>MTTVMKFGGTSVGSGERIRHVAKIVTKRKKEDDDVVVVVSAMSEVTNALVEISQQALDVRDIAKVGDFIKFIREKHYKAIEEAIKSEEIKEEVKKIIDSRIEELEKVLIGVAYLGELTPKSRDYILSFGERLSSPILSGAIRDLGEKSIALEGGEAGIITDNNFGSARVKRLEVKERLLPLLKEGIIPVVTGFIGTTEEGYITTLGRGGSDYSAALIGYGLDADIIEIWTDVSGVYTTDPRLVPTARRIPKLSYIEAMELAYFGAK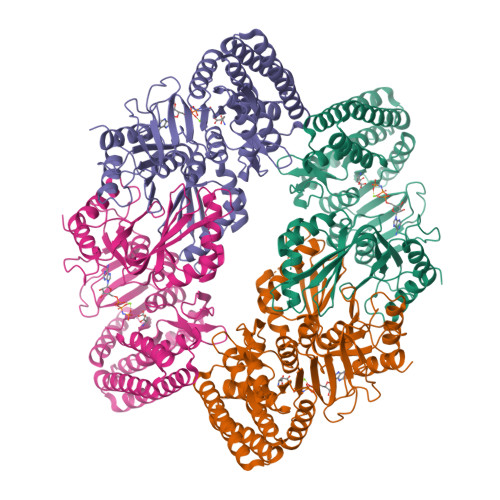VLHPRTIEPAMEKGIPILVKNTFEPESEGTLITNDMEMSDSIVKAISTIKNVALINIFGAGMVGVSGTAARIFKALGEEEVNVILISQGSSETNISLVVSEEDVDKALKALKREFGDFGKKSFLNNNLIRDVSVDKDVCVISVVGAGMRGAKGIAGKIFTAVSESGANIKMIAQGSSEVNISFVIDEKDLLNCVRKLHEKFIEKTNS[4x]> MKKLAIVALLASLHAVPALALDVPSSSRYDHRIRYVTYNPADVVQVDTVLGVATHIMLEEGEQYLTHAFGDSEAYAFARKGRHIFIKPQAELANTNLIVVTDRRSYKFRLQMRNDRNGAMYELAFRYPDTQARQTREANARAAVEAAFEQRVGAYYNLKYMMSGDKDIAPVNA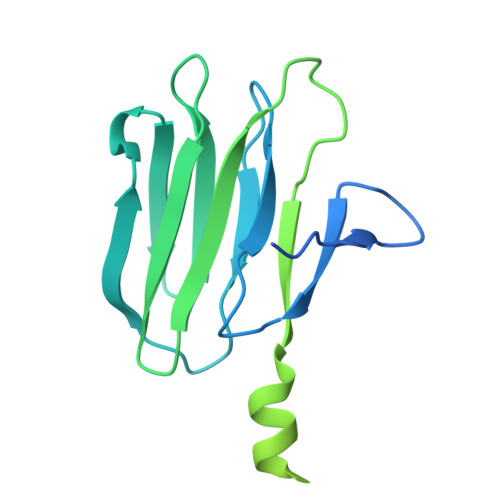WDDGRFTYFKFSANADLPSIYFVDAEGNESLVPRTTVGSSNNIIAVHKVNPKWMIRLGNRALAIFNEAYDPNGVPNDTGTASPAVRRVNKGGN2-[4-amino-1-(propan-2-yl)-1H-pyrazolo[3,4-d]pyrimidin-3-yl]-1H-indol-5-ol | C16 H16 N6 O | 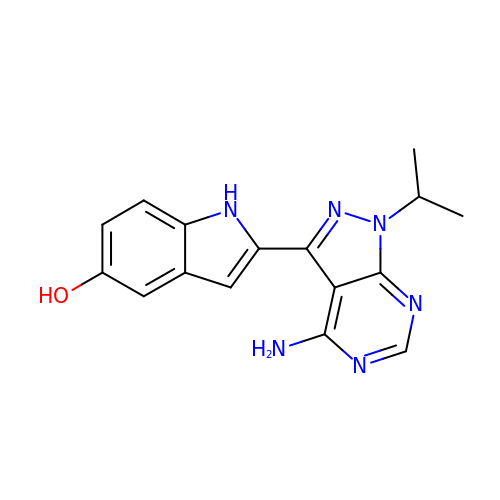MFAQYJIYDMLAIM-UHFFFAOYSA-N> MSLSRIVYVLLLFIASWSLYYLLGQEQDSKIQVAPNLELPMFSGENLENISYDEQGIRNY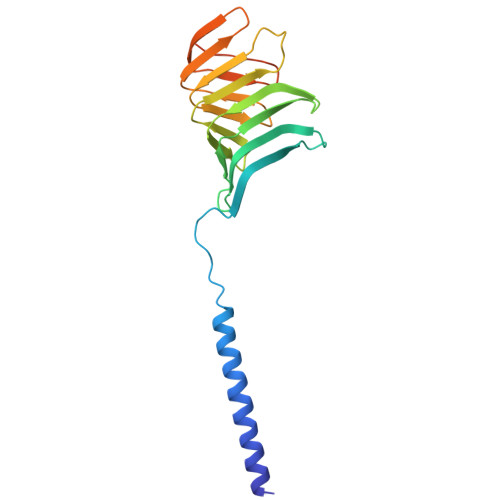VITSIHLDHYAKSGNTLFKAPILKVYREGTLQEWEITARRGILSKDQVLTLYDDVLAKNLLPDSGFDTLTTSEMSIQLKSRDFWADKPVELRGPQFETHGQAMKGNFADHSAELYNQVQGRYETLTPLVPR Herein we report the first X-ray crystal structures of mixed chirality α-helices in short peptides comprising only natural residues as the example of a stapled bicyclic and a linear membrane disruptive amphiphilic antimicrobial peptide (AMP) containing seven l- and four d-residues, as complexes of fucosylated analogs with the bacterial lectin LecB. The mixed chirality α-helices are superimposable onto the homochiral α-helices and form under similar conditions as shown by CD spectra and MD simulations but non-hemolytic and resistant to proteolysis. To get a direct insight into the structure of AMBP bp65/bp69 and their linear analogs ln65/ln69, we performed several crystallization studies using either the compounds themselves or their racemates to be crystallized as pure compounds, or their fucosylated derivatives of both mirror image peptides as complexes with the P. aeruginosa lectin LecB. While previous reports of similar mixed chirality AMPs concluded on either unordered conformations or helical conformations appearing in a membrane environment based on deconvolution of FTIR spectra, here we reported X-ray crystallographic evidence of short mixed chirality helices consisting of only natural residues existing as helix bundles within the protein environment of a lectin and almost perfectly superimposable with their parent homochiral α-helices. These direct observations unequivocally demonstrate that the α-helical fold with only natural residues can sometimes tolerate multiple stereochemical inversions without significant conformational changes.

The same was true across the ten different X-ray structures of linear α-helices observed in the X-ray structures of LecB complexes for the homochiral Fln65 and its mixed chirality analog Fdln69 (RMSD < 0.9 Å). This comparison showed that the helical geometries of the homochiral and heterochiral helices were not significantly different from each other. A similar α-helical fold was observed for the corresponding linear mixed chirality peptide ln69 and the homochiral sequence ln65. Surprisingly, the mixed chirality sequences bp69 and ln69 showed similar CD spectra and an even stronger α-helical signal as their homochiral parents in 5 mM DPC although they contained 7 l- and 4 d-residues (ESI†). To test whether the α-helix was stabilized by the bicyclic staple, we repeated the MD simulation with linear analogs ln65 and ln69, which again showed rapid unfolding in water but refolding to a stable α-helix at the DPC micelle surface for both the homochiral linear peptide ln65 and the mixed chirality linear peptide ln69. The mixed chirality linear AMP ln69 showed comparably strong antibacterial activities but reduced hemolysis and much stronger stability against serum proteolysis compared to its homochiral parent ln65, similar to previous reports with mixed chirality AMPs.

>[4x]MATQGVFTLPANTRFGVTAFANSSGTQTVNVLVNNETAATFSGQSTNNAVIGTQVLNSGSSGKVQVQVSVNGRPSDLVSAQVILTNELNFALVGSEDGTDNDYNDAVVVINWPLG;>KKLLKLLKLLLX[4x]> SKNKEDKRNAEYRLAFEQLNFVGADSKTPILKSFIEDKGTRIDEITFESMIPIETWKSYIPQLQTSLNISIISIEQGASKRIVIIKSMAGDAKIPKYLPWDDKYIEEQEGVVVVGQTFSGNIKIDLNKSPHILSAGETGSGKSVILRCILWQLLKQGAIAYMVDFKGGVEFGLEYEKVGQVITEVDAAEKLFKYLVDENAKRLKLLRESGSKNIGEYNKKFEGEELKRIIVVIDELAELMDKTGVDDETRAKLVRIEGYTSTLARLSRATGINLCIGVQRPDAKVITGQIKNNVPVRICGRFADSKASEIVLSNTKAKDLPEVKGRFLFKLGADTVQ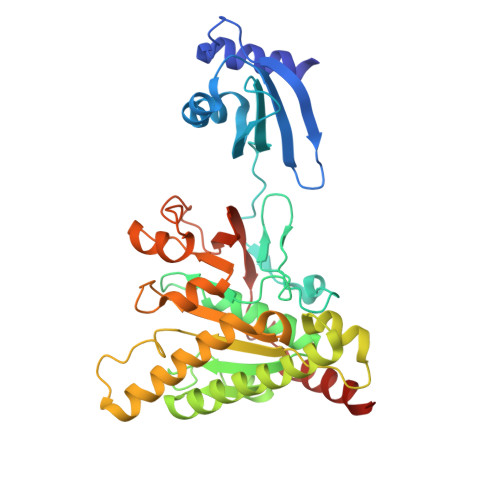FQAFYFDDDKHFIPNKILKLRKDEIEDK In R. marinus, ACIII is composed of seven subunits encoded by the Act gene cluster, six of which are conserved across species (ActA to ActF). ACIII is composed by a combination of proteins present in other respiratory complexes, which reinforces the modularity concept of energy transducing machines. Our structure shows that ACIII meets all requirements for an energy-transducing machine that couples quinol oxidation to translocation of protons across the membrane.

In this work, we describe a 3.9 Å cryo-EM structure of ACIII from R. marinus. ACIII is an L-shaped complex of ~130 Å by ~110 Å with a membrane domain and two peripheral domains facing opposite sides of the membrane. The structure shows that ACIII subunits are organized into two functional modules: (i) the electron transfer module, composed of subunits ActA, ActB, ActE, ActH, and one unidentified subunit and (ii) a module for membrane attachment, quinol-binding and ion translocation, comprising membrane subunits ActC, ActD, and ActF. Subunits ActA, ActB, and ActE in the large peripheral domain accommodate all the prosthetic groups in the complex, for a total of six hemes and four iron–sulfur clusters. The putative quinol-binding site is located at the periplasmic side of the membrane, in the first four-helix bundle of ActC, at a distance of 10–12 Å from cluster FeS1 in ActB. The location of the quinol pocket also agrees with the quinol-binding site of the homologous PsrC, identified by co-crystallization experiments, with a C-alpha RMSD at the periplasmic side of the first four-helix bundle of 1.446 Å. Heme I is more than 20 Å away from the putative quinol-binding pocket, suggesting that FeS1 is the primary electron acceptor from the quinol. Analysis of the ITC data revealed an ideal fitting by a 1:1 binding model and a binding constant (log Ka) of 6.5 ± 0.14, supporting our observation of a single quinol-binding site in ACIII. The observation of two likely proton pathways suggests the existence of two proton-pumping sites in ACIII. Interestingly, Glu122D is placed together with the conserved residues Ser245C and Tyr284F in a plane parallel to the membrane that coincides with the position at which the proton half-channels in ActC and ActF converge.

> MPQIFSRKTNRLPALSLAGSVFGGVLAVFLVWYYFSPEFYEVGYAPPYSHRIHVGKLGLDCRYCHNWVEVSDKANIPPTQTCINCHSQILTDSPRLQAVRDSWATDRSIEWVKVHHLPDYAHFSHASHVNNGVGCETCHGRIDQMDVVRLVEPLSMGWCLECHRQPELYLRPQSEITTMGYQPPADYIERNLERIRKEGIRPPTNCSACHY;> MIELPVVNPDGAETPGSGKRLWRSTADLRRDPEWVKLAHDEFMPGVAEPPSGTSRRQFLQIMGASMALAGLTACRRPVEKILPYVRQPEEIIPGIPLYYATAMPFRGSVRPLLVESHEGRPTKIEGNPDHPLSRGATGVFEQASLLNLYDPDRSQQVLRKGEPASWGDFVQFARSLAAEAGTKRLAVLCEPSSSPTLAALRRELERRYAQVRWVTYRPEGDDHEALGLQQAFGRPVRARYRFSEARVIVSLDADFLGPTDRNFVENTREFAASRRMERPEDEISRLYVIESTYTVTGGMADHRLRLRAGDIPAFAAALAAELGVGELREAGARFAGHPYVVEIARDLRAAGARGVVLAGETQPPAVHALCAVINDLLGSLGRTVILHALDEPATAQHAALAELVQAMQAGAVDALLLLNVNPVYDAPAALGFAEALAQVPEVIHLGLHVDETARRSTWHLPSTHYLEAWGDGRAYDGTLSVIQPLIAPLYEAAHSPLEVLALLATGEEQSAYDLVRNTWRRLLAGRGAFEQAWQRVLHDGFLPDSGYPTVSLRPNRQALADWPQAAEGGLEVVFRLDPTVLDGSFANNAWAQELPDPITKIVWDNVAILSPKTAAALGVKAEYHKGVYIADVIELSLDGRAVELPVWVLPGHPDDSITVYLGYGREITSTRPERKTPFFDLDDYTDIYGHGAIATGVGVNVAPLRRPDNTWVAYGAQVRKTGRTYKIVTTQDHGSMVGRPLVRLATVEEFRKNPDFAKEAEPPLEGLEPWDQYPTLWEENHPSKQPAFQDSDYYRNQWAMVIDLNACTGCNACIVACDSENNIPMVGKNEVGRGREMHWLRIDRYFVSDEAHADDPQIVVQPVPCMHCENAPCESVCPVAATVHSPDGLNEMVYNRCIGTRYCSNNCPYKVRRFNWFNWVKTLPIQVQMAQNPDVTVRFRGVMEKCTYCVQRIREAQRQANIEKRPLRDGEVKTACQQACPAEAITFGDLNDPNNAVVKQRQNARRYEMLAALNVKPRTSYLARITNPNPRLLEQEPVA;> MAHATKDLSALARTDEEVLVQGGLTFHDITELVAQHTEKKTPKAWWAAFSVAFLGMLTLVAMLAYQVWNGVGVWGNNIPVGWGWPIVNFVFWVGIGHAGTLISAILFLFRQRWRTSINRAAEAMTIFAVICALIFPTFHVGRVWAIYWTLPIPNQMEMWPQFKSPLLWDVFAVSSYFIVSLVFWYVGLIPDLATLRDRAALMGRRLRAKILGFFALGWCGANRHWRNYEKVYMLLAGLATPLVLSVHSVVSFDFAVSIIPGWHTTIFPPYFVAGAIFSGFAMVVTLMVIARKAYGLENVITIDHLEKMNIIMLVTGTMVGFAYITEFFIAWYSGVPYEQYAFINRATGPYAWAYWTMMSCNLIFPQFFWIKKLRRNIPFMFIASIVVNIGMWFERFVITITSLHRDYLPSSWDYFVPTWVDVLTLIGSFGLFFTLFLLFLRFVPMVAIAEVKGVLPEADPHFYETHGDGHSRPAEVQVNRGRSS;> MLKELLRSLKASMGIYEARDGSIYGLLAEFSDPAALLHAARQVRKAGYRHFDAHSPFPIHGMDEAMGLGNSKVAFITFFTGTIAGFALAWWMQWWMGAVDYPLNISGKPFFALPPSVPIIFELTILFSALAGVATMLALNGLPRPYNPLFYSKNFMRVTDDGFFLFVAASDPKFDPTATRQLLEQLGGYNIEVIEDRGEEDVTPATAPAAEAAVTTS;> MQNITAMPRTIWTGLLLGLLLAGCRGMISSKPPVHPNLNMDFQEKFEAQELNPFFADRRAMRPPVPGTVPRGLLKEDTPFYFGKTADGAYVERIPVAVTPELVARGRERYNIYCAVCHGQAGDGQGIIMRGNYGYTPAPSFHDDRLRNVEDGYIFDVISHGVRNMPAYGHQIPVADRWAIVAYVRALQRSQHATAADVPEEVRARLQGE;> MAEVKANGFPGWLLDPLRPTREKAEPRYRLPEDVRIWAVPLAIGVGLLIVSLVGWAIDARQFYFSYLVGWTFCLTLALGSLFFVMIQHLTRAQWVVAVRRLPEALVWTFPVLIVLFIPILFGLHDLYHWTHHELYDPSSPEYDPILAGKHAYLNVPFFLVRIAFYFFIWTLLAYKLYTLSVRQDVDPDPSIPAQQRKVSAWGMPLYGVTVAFASYDFLMSLDPHWYSTIFGVYFFAGSFFVALGFITTCYAILVRRGTLQGIVRAPHFQDLGKLMFGFTAFWAYIAFSQYMLIWYGNLPEETLWYRHRLEHGWEVLSQVLIWGHFVLPFLILLPWAAKRTPVLVGTMGIWFAIIHWIDLFWVAMPVLHTEHMTFHWLDVTCWLGLFGVVVGLFFYRISRHSLVPQNDPYLARSLALH;> MKRYPGLIGLLVVLVSVAGCRFYGYPGGVALTLAQIEAASEQVAQDLEQALAELEALRLLARRDETLAPYVAQYEAILEAHQQAVLEFEHWKEQVAAHPGDYRRANRTLGAITARHEALLQQYADVAWAVAQHVNPALLARAYTSSGPRFFFYVVPPQYARQVNEQAVPPLQVVRYLAAQLS>[4x]MKFTLLSVVAIAAAASDSYAAPAASSLAGPVTTGVFSAVSAIPSFATNLSGQVASATSTVLSGSTASGSSATAAPSASASGASSMQSMASSLSG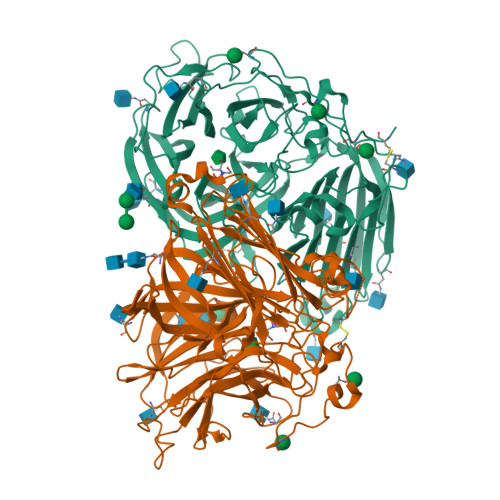SAFSPSSMMPIASGNMTMPNMTSSASASSAASTATGVAGGAGSNSSSSCAPTSLPASATELPTTVPTGTVITGDYTGSYRPQVHYSPPKGFMNAPNGCHRDRNGTYHLYYQYNPLEYVAGNQHWGHATSDDLYHWTNQPIAIFPPNSTSQVFSGSAVLDPNNTSGFFPNTTDGVVAVYTLNTPTLQVQEVAYSTDGGYNFTPYENNPVLSVGSNQFRDPKVFWYEDHWVMAVAAANDFTIEIYTSPNLTSWTFASNFTHHGLLGLAYECPNLVQVPFQDDPSKSAWLMYISINPGAPLGGSVGQYFPGDFNGTHFVAYDSAARIADFAKDNYASQWFADTENGESISIAWASNWQYTQQVPTSAQAFRSAMSLPRRNYLTNITRLGWDLVSLPYDLSPVVGPSLLSSSEANSTADVDFTNVTSNAVWFSLNVTLPDAAIQNASLISADASINITFLPSTKCSSSSGSGSDSPAATLTYFYAGLTNGALALTRPAASSSWGAENPFFTDKFSYTLVDPLTSLVGVFDRSMLEVFVNEGAHSATMLVFPDSPVGSMKVATGGLPEGTQVNLQVNGLESTWQSS>GAMGS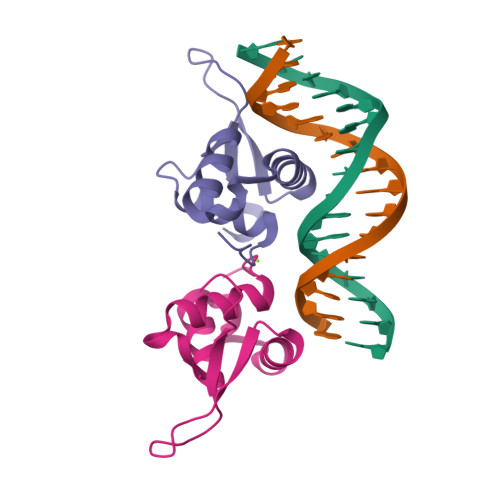HAKPPYSYISLITMAIQQAPSKMLTLSEIYQWIMDLFPYYRQNQQRWQNSIRHSLSFNDCFVKVARSPDKPGKGSYWTLHPDSGNMFENGCYLRRQK[4x]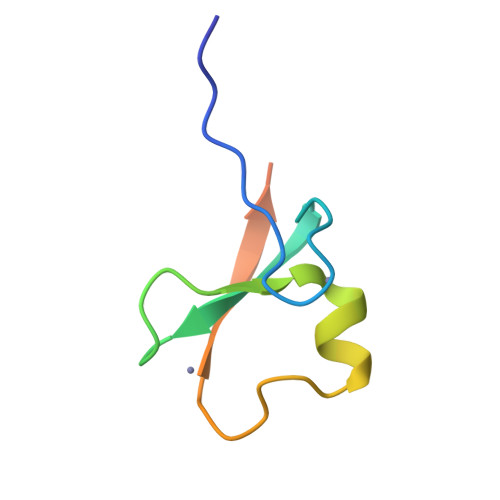>LEEEDVICDGCNGPVVGTRYKCSVCPDYDLCSVCEGKGLHRGHTKLAFPSPFGHLSEGFS[2x]Here we report cryo-electron microscopic structures of the heme translocation complex CcmABCD from E. coli, alone and bound to the heme chaperone CcmE. CcmABCD forms a heterooctameric complex centered around the ABC transporter CcmAB that does not by itself transport heme. Our data suggest that the complex flops a heme group from the inner to the outer leaflet at its CcmBC interfaces, driven by ATP hydrolysis at CcmA. A conserved heme-handling motif (WxWD) at the periplasmic side of CcmC rotates the heme by 90° for covalent attachment to the heme chaperone CcmE that we find interacting exclusively with the CcmB subunit.

Here we generated a series of expression constructs for components of the Ccm system of E. coli and isolated a CcmABCDE complex that was solubilized with DDM or GDN and isolated by affinity and size exclusion chromatography. This sample was then characterized by cryo-EM single-particle analysis, and classes representing a Ccm(ABCD)2 and a Ccm(ABCD)2E complex (see below) were refined, leading to structural models at resolutions of 3.47 Å and 3.81 Å. In our analysis, the Ccm(AB)2 unit is also at the core of the complex, but already in initial 2D classes it immediately became apparent that the assembly was symmetric, with CcmCD modules on both sides of the core transporter, resulting in a Ccm(ABCD)2 heterooctamer with a total mass of 164 kDa and 26 transmembrane helices. The ABC transporter was in a nucleotide-free, inward-open state, without direct contact between the two nucleotide-binding CcmA subunits. In all motifs, the conserved residues given in bold are involved in binding MgATP. In the nucleotide-free state of the complex there were no direct interactions between the two copies of CcmA, their centers of mass were 36 Å apart. The overall architecture of the CcmABCD complex in its nucleotide-free state thus is a C2-symmetric heterooctamer with dimensions of 100 Å × 80 Å × 60 Å. It contains a pronounced groove between the CcmB, CcmC and CcmD subunits on either side that is capped by the WxWD loop of CcmC at the periplasmic interface. For the following discussion, we designate this face of the complex the ‘front’ and the opposite side, with a rather flat CcmBC interface, its ‘back’. Most obviously, we have isolated a heterooctameric Ccm(ABCD)2 complex as a predominant species in the nucleotide-free state, while the structures reported previously consistently only contained one copy each of CcmC and CcmD. No bound heme was found in the structural analyses of different complexes, while heme-bound structures were obtained in the recent report on a Ccm(AB)2CD complex, but here external hemin was added prior to cryo-EM analysis. We had not followed this strategy, and this presumably led to the loss of the non-covalently bound cofactor during grid preparation.

>[2x]MASWSHPQFEKMGMLEARELLCERDERTLFSGLSFTLNAGEWVQITGSNGAGKTTLLRLLTGLSRPDAGEVLWQGQPLHQVRDSYHQNLLWIGHQPGIKTRLTALENLHFYHRDGDTAQCLEALAQAGLAGFEDIPVNQLSAGQQRRVALARLWLTRATLWILDEPFTAIDVNGVDRLTQRMAQHTEQGGIVILTTHQPLNVAESKIRRISLTQTRAA;>MMFWRIFRLELRVAFRHSAEIANPLWFFLIVITLFPLSIGPEPQLLARIAPGIIWVAALLSSLLALERLFRDDLQDGSLEQLMLLPLPLPAVVLAKVMAHWMVTGLPLLILSPLVAMLLGMDVYGWQVMALTLLLGTPTLGFLGAPGVALTVGLKRGGVLLSILVLPLTIPLLIFATAAMDAASMHLPVDGYLAILGALLAGTATLSPFATAAALRISIQ[2x];>MWKTLHQLAIPPRLYQICGWFIPWLAIASVVVLTVGWIWGFGFAPADYQQGNSYRIIYLHVPAAIWSMGIYASMAVAAFIGLVWQMKMANLAVAAMAPIGAVFTFIALVTGSAWGKPMWGTWWVWDARLTSELVLLFLYVGVIALWHAFDDRRLAGRAAGILVLIGVVNLPIIHYSVEWWNTLHQGSTRMQQSIDPAMRSPLRWSIFGFLLLSATLTLMRMRNLILLMEKRRPWVSELILKRGRK[2x];>MTPAFASWNEFFAMGGYAFFVWLAVVMTVIPLVVLVVHSVMQHRAILRGVAQQRAREARLRAAQQQEAA[2x]>[4x]NLPPEKKWLGTPIEEMRKMPRCGIHLPSLRPSASHTVTVRVDLLRAGEVPKPFPTHYKDLWDNKHVKMPCSEQNLYPVEDENGERTAGSRWELIQTALLNKFTRPQNLKDAILKYNVAYSKKWDFTALVDFWDK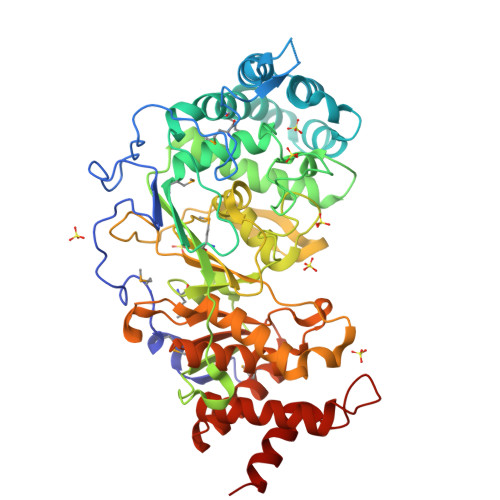VLEEAEAQHLYQSILPDMVKIALCLPNICTQPIPLLKQKMNHSVTMSQEQIASLLANAFFCTFPRRNAKMKSEYSSYPDINFNRLFEGRSSRKPEKLKTLFCYFRRVTEKKPTGLVTFTRQSLEDFPEWERCEKPLTRLHVTYEGTIEGNGRGMLQVDFANRFVGGGVTGAGLVQEEIRFLINPELIVSRLFTEVLDHNECLIITGTEQYSEYTGYAETYRWARSHEDGSEKDDWQRRCTEIVAIDALHFRRYLDQFVPEKVRRELNKAYCGFLRPGVPSENLSAVATGNWGCGAFGGDARLKALIQILAAAAAERDVVYFTFGDSELMRDIYSMHTFLTERKLDVGKVYKLLLRYYNEECRNCSTPGPDIKLYPFIYHAVESSAET>MEAKEEFAHKTLAMDVMKPRRNDPLLTVLTQDSMTVEDVETIISETTYSGFPVVVSRESQRLVGFVLRRDLIISIENARKKQDGVVSTSIIYFTEHSPPLPPYTPPTLKLRNILDLSPFTVTDLTPM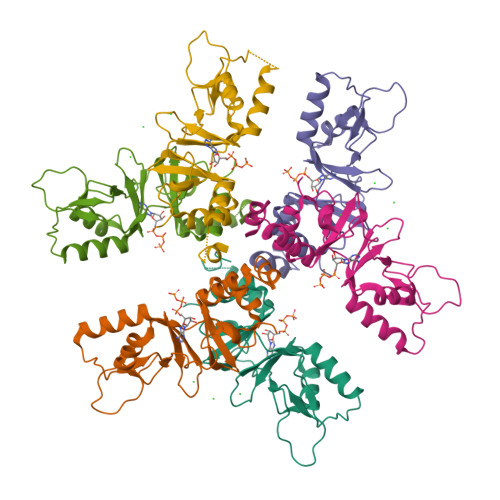EIVVDIFRKLGLRQCLVTHNGRLLGIITKKDVLKHIAQMANQDPDSILFNEFLEVLFQ[6x]> MELKEIE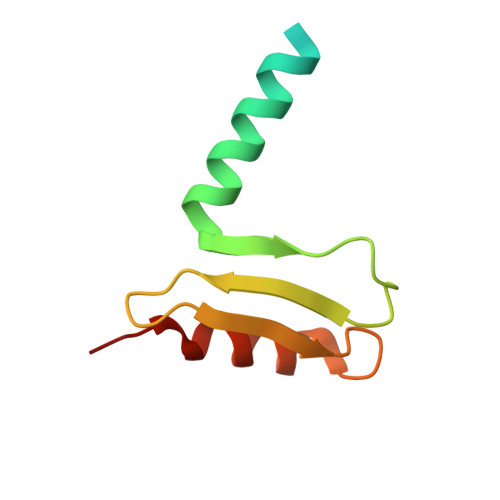ADLERQEKEVDEDTTVTIPSAVYVAQLYHQVSKIEWDYECEPGMVKGIHHGPSVAQPIHLDSTQLSRKFISDYLWSLVDTEW> MGVPAKKKQQQGERSRESILDATERLMATKGYAATSISDIRDACGLAPSSIYWHFGSKEGVLAAMMERGAQRFFAAIPTWDEAHGPVEQRSERQLTELVSLQSQHPDFLRLFYLLSMERSQDPAVAAVVRRVRNTAIARFRDSITHLLPSDIPPGKADLVVAELTAFAVALSDGVYFAGHLEPDTTDVERMYRRLR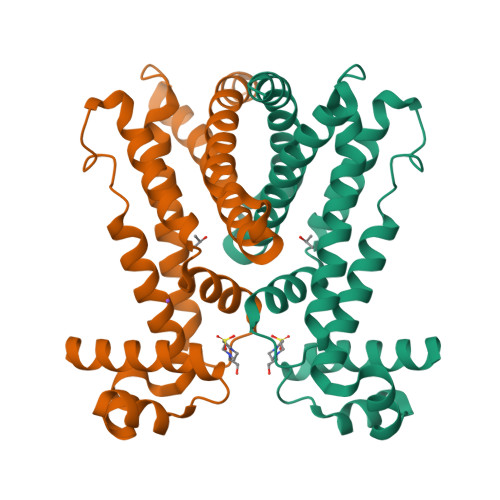QALEALIPVLLEETHHHHHH>MNPESRVIRKVLALQNDEKIFSGER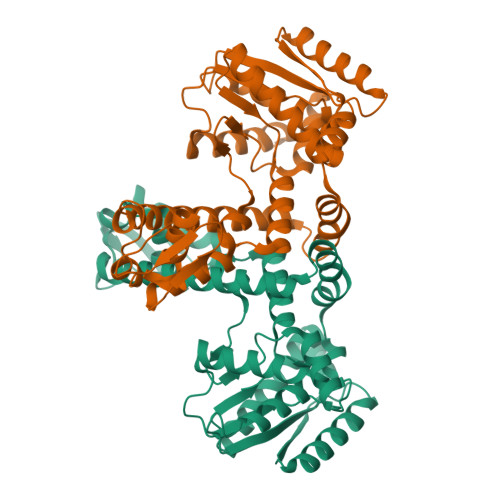RVLIAFSGGVDSVVLTDVLLKLKNYFSLKEVALAHFNHMLRESAERDEEFCKEFAKERNMKIFVGKEDVRAFAKENRMSLEEAGRFLRYKFLKEILESEGFDCIATAHHLNDLLETSLLFFTRGTGLDGLIGFLPKEEVIRRPLYYVKRSEIEEYAKFKGLRWVEDETNYEVSIPRNRIRHRVIPELKRINENLEDTFLKMVKVLRAEREFLEEEAQKLYKEVKKGNCLDVKKLKEKPLALQRRVIRKFIGEKDYEKVELVRSLLEKGGEVNLGKGKVLKRKERWLCFSPEV[2x]{[(1R,3S,4S,5R,6S)-2,4,5,6-tetrakis(phosphonooxy)cyclohexane-1,3-diyl]bis[oxy(2-oxoethane-2,1-diyl)]}bis(phosphonic 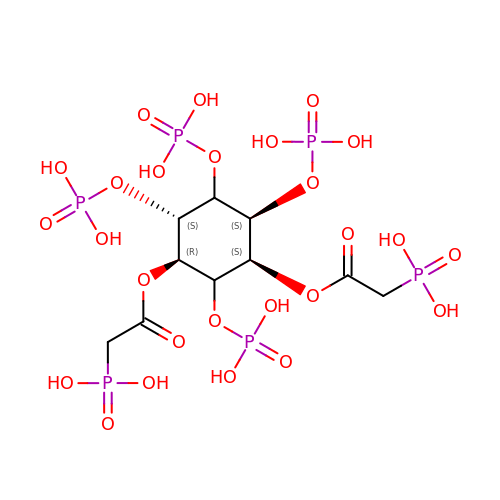acid) | C10 H22 O26 P6 | KMLKNZLYFKMCMH-COQVWMOOSA-N>[4x]GPMTADAPAGTLAQPGGISDPNLIKLVNKLQDVFTTVGVNNPIDLPQIVVVGSQSSGASSVLENIVGRDFLPRGQGIVTRRPLVLQLINRQSSGNANGFDERLADSTDKAANLDEWGEFLHLP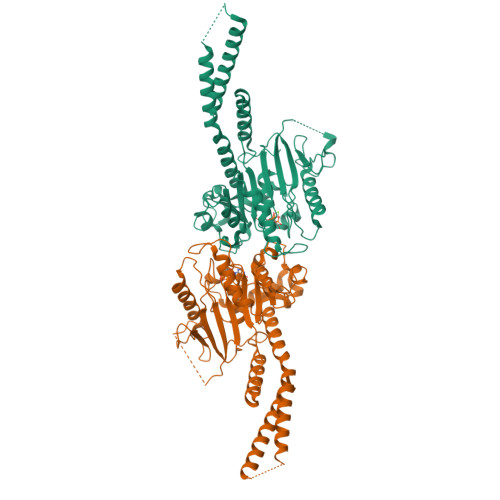GQKFYDFNKIRDEINRETEAKVGRNAGISPAPINLRIYSPHVLNLTLVDLPGLTRVPVGDQPRDIERQIRDMILKYIQKPNAIILAVTAANVDLANSDGLKLAREVDPEGQRTIGVLTKVDLMDEGTDVVDILAGRIIPLRLGYVPVVNRGQRDIDNKKPITAALEAEKAFFENHKAYRNKSAYCGTPYLARKLNLILMMHIKQTLPDIKQRISSSLQKYQQELEALGPSLLGAGAGAESDYTVRRRKECQQMVESLQRAAEIVSQVQ>MGSDSIDTPNYDVQKHINKLCGMLLITEDANHKFTGLIGMLYAMSRLGREDTIKILRDAGYHVKANGVDVTTHRQDINGKEMKFEVLTLASLTTEIQINIEIESRKSYKKMLKEMGEVAPEYRHDSPDCGMIILCIAALVITKLAAGDRSGLTAVIRRANNVLKNEMKRYKGLLPKDIANSFYEVFEKHPHFI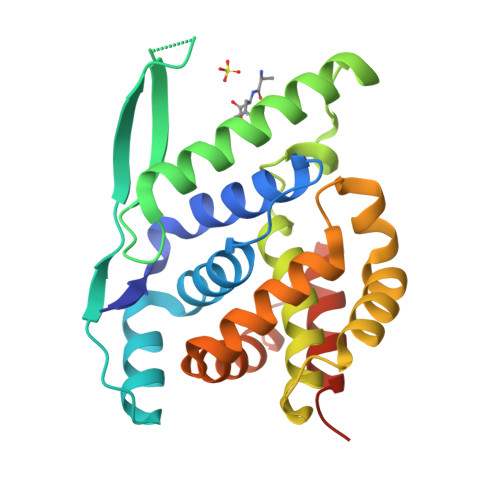DVFVHFGIAQSSTRGGSRVEGIFAGLFMNAYGLEHHHHHH[4x]>[2x]MFTGSIVAIVT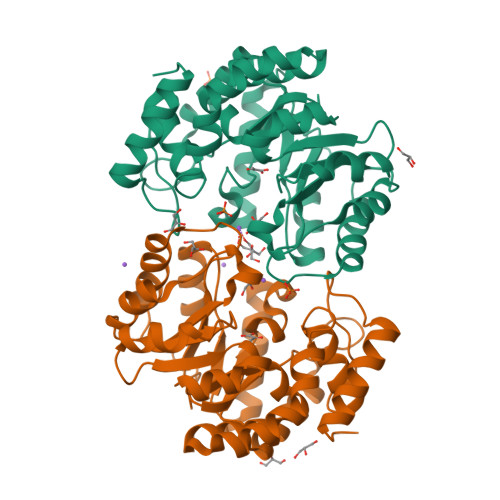PMDEKGNVCRASLKKLIDYHVASGTSAIVSVGTTGESATLNHDEHADVVMMTLDLADGRIPVIAGTGANATAEAISLTQRFNDSGIVGCLTVTPYYNRPSQEGLYQHFKAIAEHTDLPQILYNVPSRTGCDLLPETVGRLAKVKNIIGIREATGNLTRVNQIKELVSDDFVLLSGDDASALDFMQLGGHGVISVTANVAARDMAQMCKLAAEGHFAEARVINQRLMPLHNKLFVEPNPIPVKWACKELGLVATDTLRLPMTPITDSGRETVRAALKHAGLL>[2x]KVNQNQAKRCTVIGGSGFLGQHMVEQLLARGYAVNVFDIQQGFDNPQVRFFLGDLCSRQDLYPALKGVNTVFHCASPPPSSNNKELFYRVNYIGTKNVIETCKEAGVQKLIL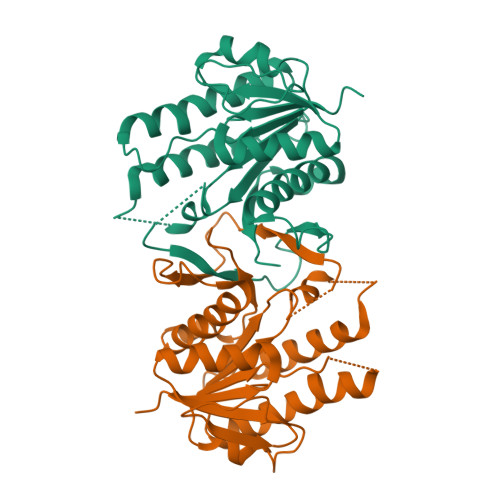TSSASVIFEGVDIKNGTEDLPYAMKPIDYYTETKILQERAVLGANDPEKNFLTTAIRPHGIFGPRDPQLVPILIEAARNGKMKFVIGNGKNLVDFTFVENVVHGHILAAEQLSRDSTLGGKAFHILEHHHHHH Podophages that infect gram-negative bacteria, such as Pectobacterium pathogen ΦM1, encode tail assemblies too short to extend across the complex gram-negative cell wall. To overcome this, podophages encode a large protein complex (ejectosome) packaged inside the viral capsid and correspondingly ejected during infection to form a transient channel that spans the periplasmic space. Here, we report a near-complete atomic model of the bacteriophage ΦM1.

Bacteriophage ΦM1 encloses the viral DNA within a highly decorated T = 7 icosahedral capsid composed of HK97-like major capsid proteins (MCPs) and two similar, but distinct, accessory proteins. Two decoration proteins, gp44 and gp43, are individually expressed off the viral genome and bind across MCPs at the 2-fold and quasi-2-fold axes of symmetry via formation of homodimeric α-helical bundles, where each dimerization domain consists of a helix–turn–helix motif. We refer to these bundle structures as α-claw motifs, as corresponding density bears resemblance to claw clips. The gp44 consists only of the α-claw motif, which we refer to as the α-claw protein. Gp43, however, also encodes a long helical fiber that we term the “forearm” domain. We refer to gp43 as the α-paw protein. While the α-claw is a small protein (∼6 kDa) and is composed primarily of two α-helices, the α-paw is nearly three times the size (∼17 kDa), due to the long C-terminal forearm domain. The α-claw and α-paw decoration proteins, although similar in the helix–turn–helix domain, may serve different functions during infection by virtue of their structures. Both decorations likely stabilize the capsid as they bind across MCPs, which is a common function for accessory proteins in large capsid viruses which can reach up to 60 atmospheric units of internal pressure once packaged. Given that the α-claw appears to form a stronger interface with MCPs and does not encode any additional fiber, we hypothesize that this protein is required to maintain capsid stability. In contrast, the α-paw likely contributes to stability to a lesser extent but may mediate additional functions via the fibrous α-paw forearm domain, such as host recognition and adhesion.

>MSDTPYKADLSRVHWAGSNSDVDIHLEIFEGDVDSGFMYNSFFRGNSSYVSVQDQSNQARIDRMNTVTIKGRTPGQKLDRESVKNDKLVITVDTVTYASTVMDWQDDWTSPDRWAEIGAQHGYQHARLFDTAHLIQIIKARKWIAPADLKPAFFDGKEYTAAYNADRELFAANIIDAHRQGIEEMVRRDLGGSLTEFITVVSPYVFGLLLDSKKLVNVDYSAGNGNFAERRVGMVNGVRIVESARFPAAAGTSPLGAAFTVDADDVACQMVVYHPKMTLVTVEAKPLATNKYPDNPNFSDILDSFTLYTVGQRRPDTSFAVKLTNLP[7x];>MAITTGTTEAQALNMTMRDAVLKVAPGVQQLVQNSSQLTAAEIAIIQTNITALKAAFTAAGA[5x];>[2x]MSLVTATAAQRIALRNTATNLSEQTQVYAQSATAPTAAEAAIVQPYIDAAQAAITAVGAGGATVANGATVAVVNSASADSHNATATVTGTTLTNVKLAATVAFVDNADTITVQNSAGTAVAGTHTATVAAGVISNVKLAATIAPVASGLALTGVTPTGTYTNTVTFTVAAGVITAIVLS>[2x]EFSRKTYTLTDYLKNTYRLKLYSLRWISDHEYLYKQENNILVFNAEYGNSSVFLENSTFDEFGHSINDYSISPDGQFILLEYNYVKQWRHSYTASYDIYDLNKRQLITEERIPNNTQWVTWSPVGHKLAYVWNNDIYVKIEPNLPSYRITWTGKEDIIYNGITDWVYEEEVFSAYSALWWSPNGTFLAYAQFNDTEVPLIEYSFYSDESLQYPKTVRVPYPKAGAVNPTVKFFVVNTDSLSSVTNATSIQITAPASMLIGDHYLCDVTWATQERISLQWLRRIQNYSVMDICDYDESSGRWNCLVARQHIEMSTTGWVGRFRPSEPHFTLDGNSFYKIISNEEGYRHICYFQIDKKDCTFITKGTWEVIGIEALTSDYLYYIS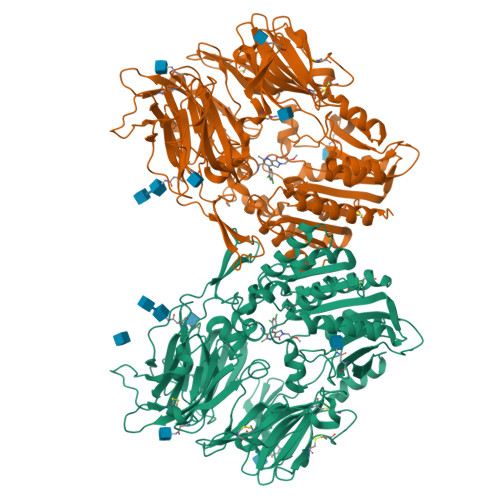NEYKGMPGGRNLYKIQLSDYTKVTCLSCELNPERCQYYSVSFSKEAKYYQLRCSGPGLPLYTLHSSVNDKGLRVLEDNSALDKMLQNVQMPSKKLDFIILNETKFWYQMILPPHFDKSKKYPLLLDVYAGPCSQKADTVFRLNWATYLASTENIIVASFDGRGSGYQGDKIMHAINRRLGTFEVEDQIEAARQFSKMGFVDNKRIAIWGWSYGGYVTSMVLGSGSGVFKCGIAVAPVSRWEYYDSVYTERYMGLPTPEDNLDHYRNSTVMSRAENFKQVEYLLIHGTADDNVHFQQSAQISKALVDVGVDFQAMWYTDEDHGIASSTAHQHIYTHMSHFIKQCFSLPPLEQKLISEEDLNSAVDHHHHHH>GTENLYFQSMDELLRRAVPPTPAYELRAATPAPAEGQCADFVSFYGGLAETAQRAELLGRLARGFGVDHGQVAEQSAGVLHLRQQQREAAVLLQAEDRLRYALVPRYRGLFHHISKLDGGVRFLVQLRADLLEAQALKLVEGPDVREMNGVLKGMLSEWFSSGFLNLERVTWHSPCEVLQKISEAEAVHPVKNWMDMKRRVGPYRRCYFFSHCSTPGEPLVVLHVALTGDISSNIQAIVKEHPPSETAAANKITAAIFYSISLTQQGLQGVELGTFLIKRVVKELQREFPHLGVFSSLSPIPGFTKWLLGLLNSQTKEHGRNELFTDSECKEISEITGGPINETLKLLLSSSEWVQSEKLVRALQTPLMRLCAWYLYGEKHRGYALNPVANFHLQNGAVLWRINWMADVSLRGITGS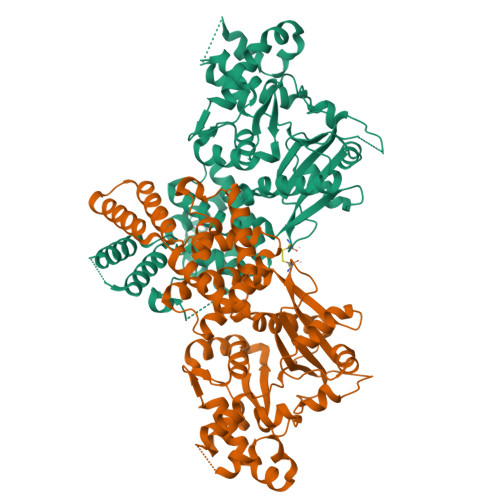CGLMANYRYFLEETGPNSTSYLGSKIIKASEQVLSLVAQFQKN[2x]>[12x]SAPADYFRILVQQFEVQLQQYRQQIEEL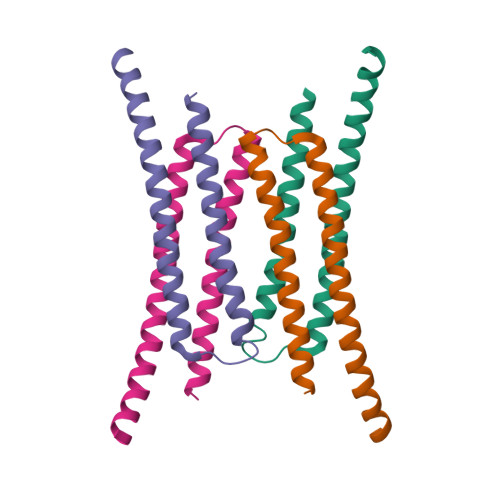ENHLATQANNSHITPQDLSMAMQKIYQTFVALAAQLQSIHENVKVLKEQYLGYRKMFL>MLMVVPLSEMGPGDKGIVVNILGGHNARQKLVSMG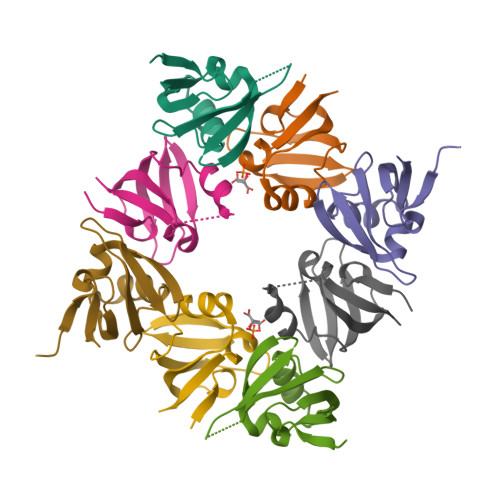LTPGATIQVLESHPMGPIIISVGGVRFAIGKGLAGRVMVRKL[4x]> MRGSHHHHHHGMASMAMYQNMLVVIDPNQDDQPALRRAVYLHQRIGGKIKAFLPIYDFSYEMTTLLSPDERTAMRQGVISQRTAWIREQAKYYLEAGVPIEIKVVWHNRPFEAIIQEVIAGSHDLVLKMAHQHDRLEAVIFTPTDWHLLRKCPSPVWMVKDQPWPEGGKALVAVNLASEEPYHNALNEKLVKETLQLAEQVNHTEVHLVGAYPVTPINIAIELPEFDPSVYNDAIRGQHLLAMKALRQKFSIDEKVTHVEKGLPEEVIPDLAEHLQAGIVVLGTVGRTGLSAAFLGNTAEQVIDHLRCDL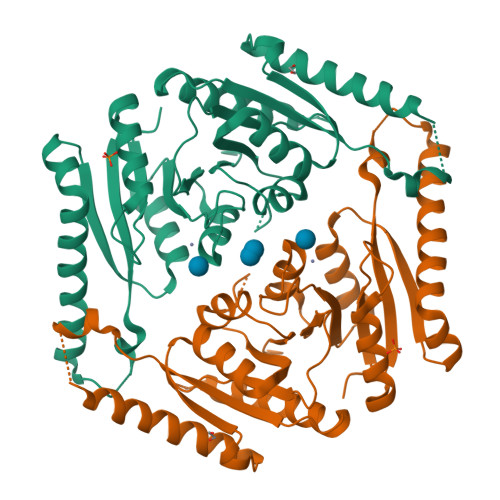LVIKPDEYQTPVELDDEDD> QIGWRREGIKYRRNELFLDVLESVNLLMSPQGQVLSAHVSGRVVMKSYLSGMPECKFGMNDKIVIEKQGKGTADETSKSGKQSIAIDDCTFHQCVRLSKFDSERSISFIPPDGEFELMRYRTTKDIILPFRVIPLVREVGRTKLEVKVVIKSNFKPSLLAQKIEVRIPTPLNTSGVQVICMKGKAKYK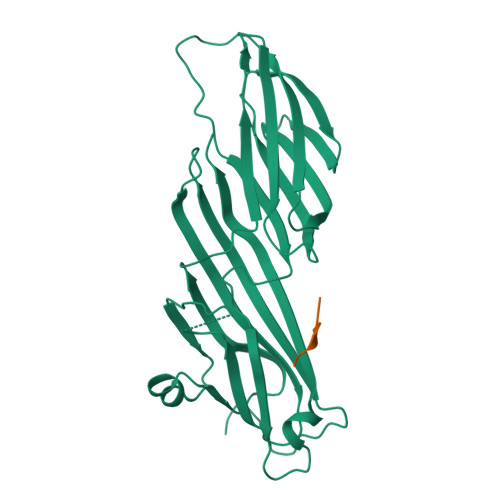ASENAIVWKIKRMAGMKESQISAEIELLPTNDKKKWARPPISMNFEVPFAPSGLKVRYLKVFEPKLNYSDHDVIKWVRYIGRSGIYETRC;> GYMMMSPS> VKELLEAGVHFGHERKRWNPKFARYIYAERNGIHIIDLQKTMEELERTFRFIEDLAMRGGTILFVGTKKQAQDIVRMEAERAGMPYVNQRWLGGMLTNFKTIQRVHRLEELEALFASPEIEERPKKEQRLHELERLQKYLSGFRLLKRLPDAIFVVDPTKEAIAVREARKLFIPVIALADTDSDPDLVDY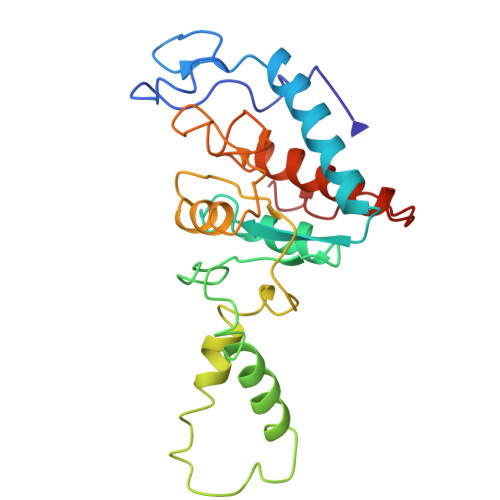IIPGNDDAIRSIQLILSRAVDLIIQARGGVVEPSPSYALVQ>[4x]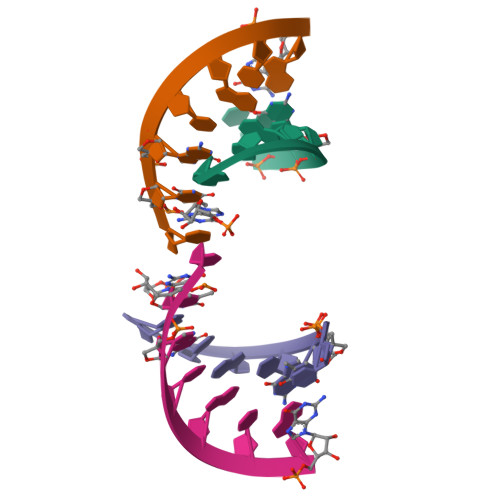NUGUACA> DEKSELSRIVRGV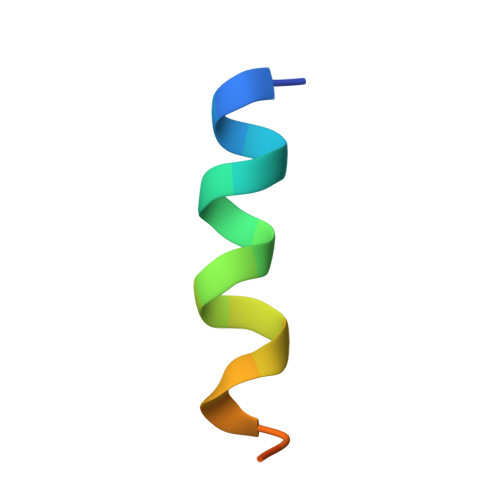QEKGPES> GSMASSSSSERWIDGLQFSSLLWPPPRDPQQHKDQVVAYVEYFGQFTSEQFPDDIAELVRHQYPSTEKRLLDDVLAMFVLHHPEHGHAVILPIISCLIDGSLVYSKEAHPFASFISLVCPSSENDYSEQWALACGEILRILTHYNRPIYKTEQQNGDTERNCLSKATTSGSPTSEPKAGSPTQHERKPLRPLSPWISDILLAAPLGIRSDYFRWCSGVMGKYAAGELKPPTIASRGSGKHPQLMPSTPRWAVANGAGVILSVCDDEVARYETATLTAVAVPALLLPPPTTSLDEHLVAGLPALEPYARLFHRYYAIATPSATQRLLLGLLEAPPSWAPDALDAAVQLVELLR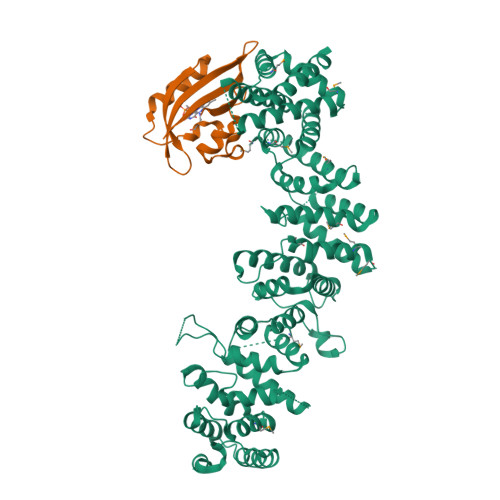AAEDYASGVRLPRNWMHLHFLRAIGIAMSMRAGVAADAAAALLFRILSQPALLFPPLSQVEGVEIQHAPIGGYSSNYRKQIEVPAAEATIEATAQGIASMLCAHGPEVEWRICTIWEAAYGLIPLNSSAVDLPEIIVATPLQPPILSWNLYIPLLKVLEYLPRGSPSEACLMKIFVATVETILSRTFPPESSRELTRKARSSFTTRSATKNLAMSELRAMVHALFLESCAGVELASRLLFVVLTVCVSHEAQSSGSKRPRSEYASTTENIEANQPVSNNQTANRKSRNVKGQGPVAAFDSYVLAAVCALACEVQLYPMISGGGNFSNSAVAGTITKPVKINGSSKEYGAGIDSAISHTRRILAILEALFSLKPSSVGTPWSYSSSEIVAAAMVAAHISELFRRSKALTHALSGLMRCKWDKEIHKRASSLYNLIDVHSKVVASIVDKAEPLEAYLKNTPVQKD;> GSNGAIPFPVGSLPGTAPCGFVVSDALEPDNPIIYVNTVFEIVTGYRAEEVIGRNCRFLQCRGPFTKRRHPMVDSTIVAKMRQCLENGIEFQGELLNFRKDGSPLMNKLRLVPIREEDEITHFIGVLLFTDAKIDLGP>SNAMLIIETLPLLRQQIRRWRQEGKRIALVPTMGNLHEGHMTLVDEAKTRADVVVVTIFVNPLQFERPDDLAHYPRTLQEDCEKLTRHGADLVFAPAAADIYPAGLEKQTYVDVPALSTILEGASRPGHFRGVSTIVSKLFNLIQPDVACFGEKD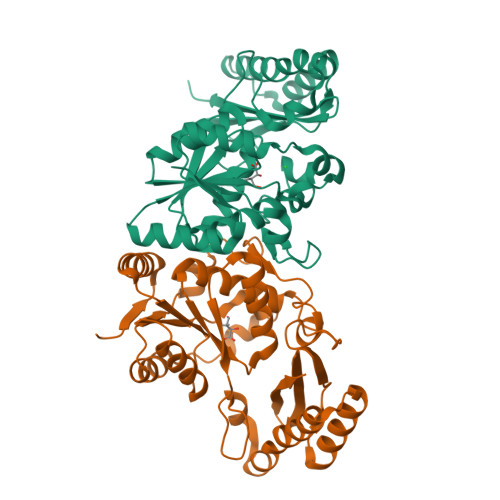YQQLALIRKMVADMGYDINIVGVPTVRAKDGLALSSRNGYLTEEERQIAPQLSKIMWALAEKMALGERQIDALLEEAAAQLLRVGFTPDELFIRDAETLQPLTVDSQQAVILMAAWLGKARLIDNQLVDLRH[4x]7,8-DIHYDRO-6-HYDROXYMETHYL-7-METHYL-7-[2-PHENYLETHYL]-PTERIN | C16 H19 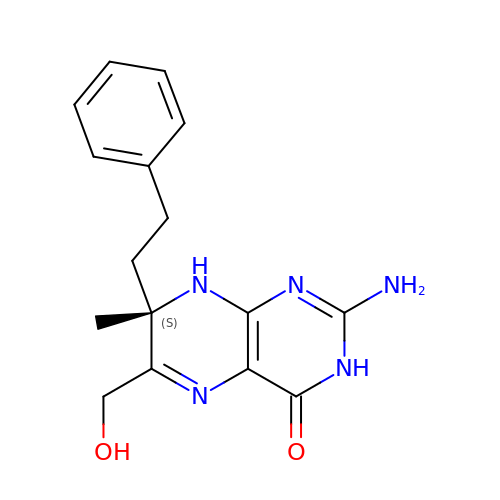N5 O2 | XMFJTCGUDFSWSW-INIZCTEOSA-N>[2x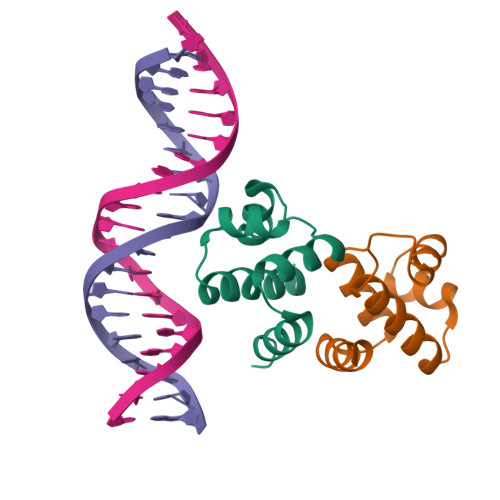]GSHMESFLLSKVSFVIKKIRLEKGMTQEDLAYKSNLDRTYISGIERNSRNLTIKSLELIMKGLEVSDVVFFEMLIKEILKHD> MPQIFSRKTNRLPALSLAGSVFGGVLAVFLVWYYFSPEFYEVGYAP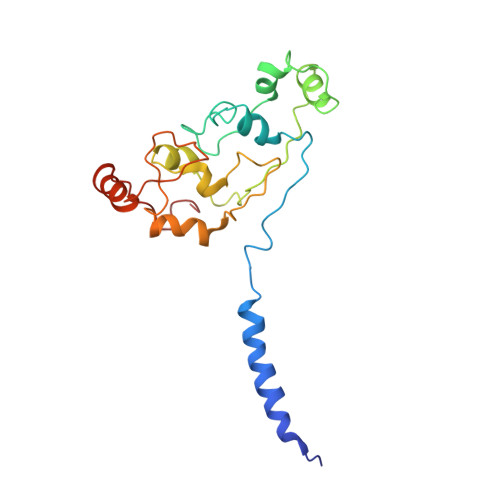PYSHRIHVGKLGLDCRYCHNWVEVSDKANIPPTQTCINCHSQILTDSPRLQAVRDSWATDRSIEWVKVHHLPDYAHFSHASHVNNGVGCETCHGRIDQMDVVRLVEPLSMGWCLECHRQPELYLRPQSEITTMGYQPPADYIERNLERIRKEGIRPPTNCSACHY> 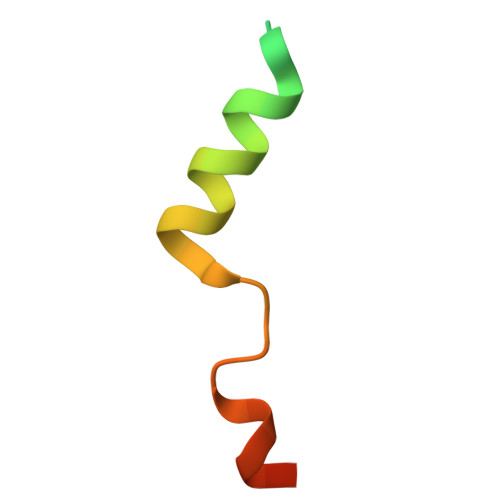GSHMREISEESISSIDYGDRDSLFFEIFGTGEEYRYVLESDP> SGSSMEGLAGYVYKAASEGKVLTLAALLLNRSESDIRYLLGYVSQQGGQRSTPLIIAARNGHAKVVRLLLEHYRVQTQQTGTVRFDGYVIDGATALWCAAGAGHFEVVKLLVSHGANVNHTTVTNSTPLRAACFDGRLDIVKYLVENNANISIANKYDNTCLMIAAYKGHTDVVR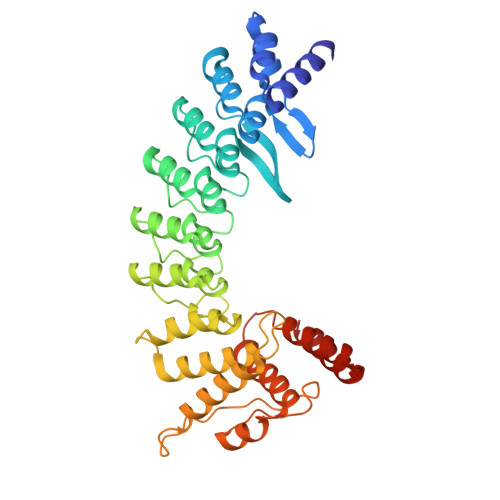YLLEQRADPNAKAHCGATALHFAAEAGHIDIVKELIKWRAAIVVNGHGMTPLKVAAESCKADVVELLLSHADCDRRSRIEALELLGASFANDRENYDIMKTYHYLYLAMLERFQDGDNILEKEVLPPIHAYGNRTECRNPQELEAIRQDRDALHMEGLIVRERILGADNIDVSHPIIYRGAVYADNMEFEQCIKLWLHALHLRQKG>[2x]TNKPIVLSTWNFGLHANVEAWKVLSKGGKALDAVEKGVRLVEDDPTERSVGYGGRPDRDGRVTLDACIMDENYNI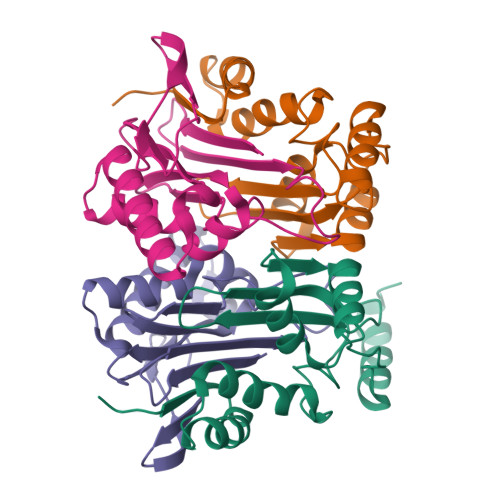GSVACMEHIKNPISVARAVMEKTPHVMLVGDGALEFALSQGFKKENLLTAESEKEWKEWLKTSQYK;>[2x]TIGMIALDAQGNLSGACTTSGMAYKMHGRVGDSPIIGAGLFVDNEIGAATAIGHGEEVIRTVGTHLVVELMNQGRTPQQACKEAVERIVKIVNRRGKNLKDIQVGFIALNKKGEYGAYCIQDGFNFAVHDQKGNRLETPGFALK>GHMIKICIAGKNNIAVNSLQFILKNYFEADQIVVIPNKNDKGIDSWQKSLLKFALDNNIKIVTLDEIYNIEQIIFFSLEFDQIIKIENFKSDRLFNIHFSALPKYKGVFTSITPILNNELESGVTLHRIDNGIDTGNIIDQH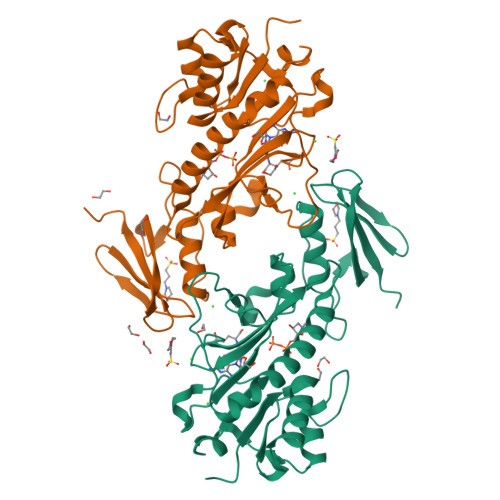CFPIDINDTARDLYFNYLKYGESIFKKNIQTIINNSYKDLKQTNINSSYFSRKDINLVHKINFKKTSFEIHNQIRAFIFQEYQLPIINNSKIIKSILANEFIGYNVFEEFENYFIISGIDGFKIIAQKLNKL[2x]> E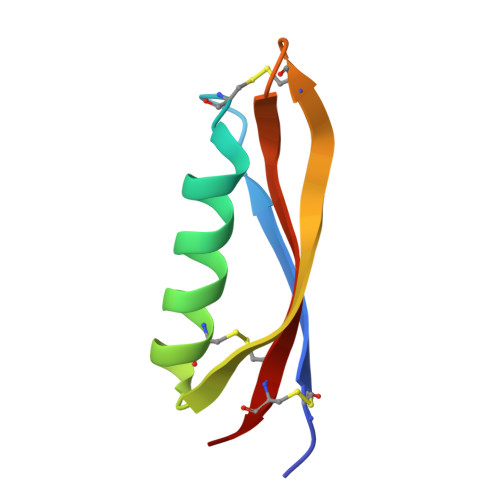ACKFLHQERMDVCETHLHWHTVAKETCSEKSTNLHDYGMLLPCGIDKFRGVEFVCCPL> HHHHHHHHGSGAGWSHPQFEKGGSGLVPRGSGSVPAGAKCRLVETLPENMDFRSDHLTTFECFNEIITLAKKYIYIASFCCNPLSTTRGALIFDKLKEASEKG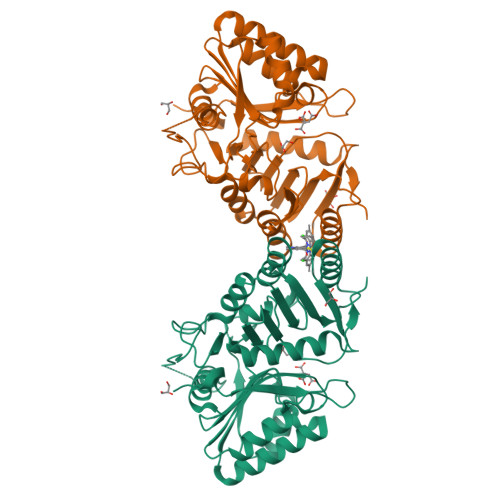IKIIVLLDERGKRNLGELQSHCPDINFITVNIDKKNNVGLLLGCFWVSDDERCYVGNASFTGGSIHTIKTLGVYSDYPPLATDLRRRFDTFKAFNSAKNSAANLASAAAALPVSTAYHIKNPIGGVFFTDSPEHLLGYSRDLDTDVVIDKLKSAKTSIDIEHLAIVPTTRVDGNSYYWPDIYNSIIEAAINRGVKIRLLVGNWDKNDVYSMATARSLDALCVQNDLSVKVFTIQNNTKLLIVDDEYVHITSANFDGTHYQNHGFVSFNSIDKQLVSEAKKIFERDWVSSHSKSLKI> MAEDFVSENSNNKRAPYWTNTEKMEKRLHAVPAFNTVKFRCPAGGNPMPTMRWLKNG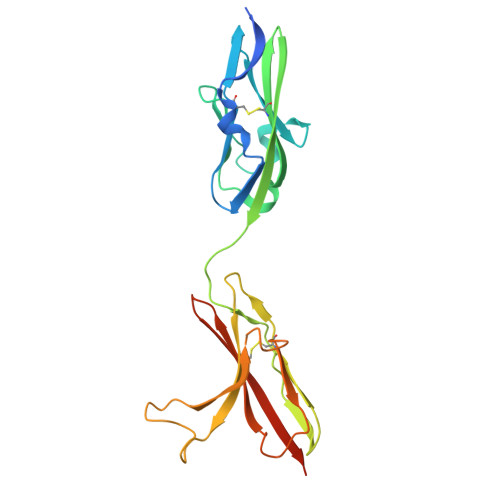KEFKQEHRIGGYKVRNQHWSLIMESVVPSDKGNYTCVVENEYGSINHTYHLDVVERSPHRPILQAGLPANASTVVGGDVEFVCKVYSDAQPHIQWIKHVEKNGSKYGPDGLPYLKVLKHSGINSSNAEVLALFNVTEADAGEYICKVSNYIGQANQSAWLTVLPKQQAPGREKE> GSHNADLSEALREL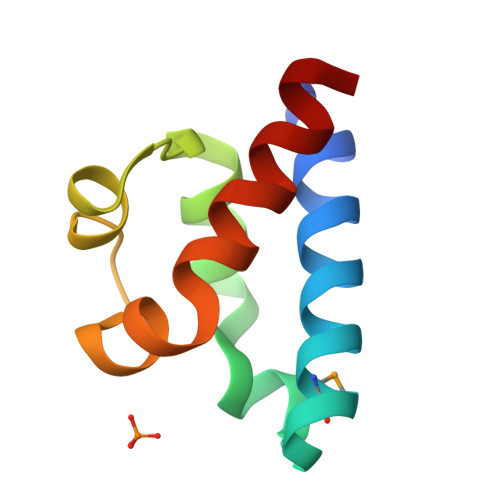RRELMKETGYSAFVVFTNATLEALAARQPRTLAELAEVPGLGEKRIEAYGERILDAINTVLDG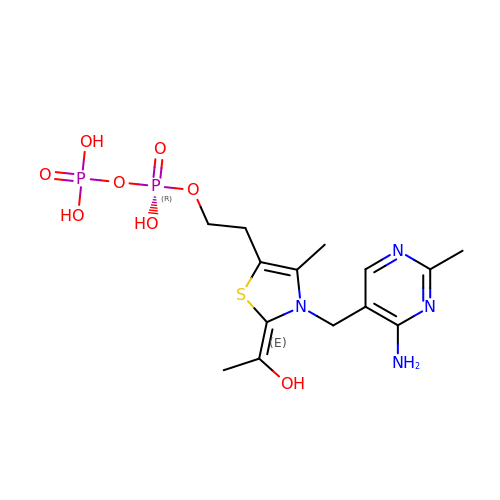2-[(2E)-3-[(4-AMINO-2-METHYLPYRIMIDIN-5-YL)METHYL]-2-(1-HYDROXYETHYLIDENE)-4-METHYL-2,3-DIHYDRO-1,3-THIAZOL-5-YL]ETHYL TRIHYDROGEN DIPHOSPHATE | C14 H22 N4 O8 P2 S | ZZLCKFKIIVXBQU-NTEUORMPSA-N> SK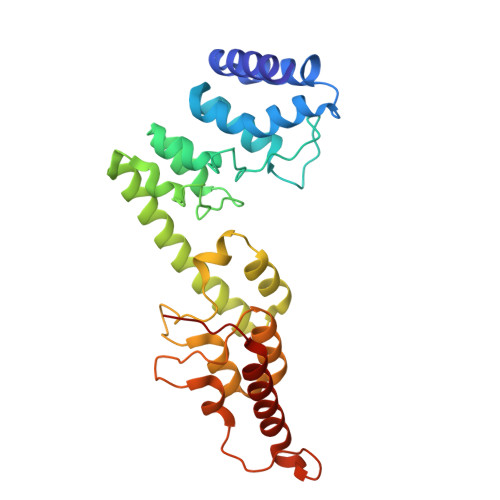PLLKLKLLDALRQGSFPNLQDLLKKQFQPLDDPNVQQVLHLMLHYAVQVAPMAVIKEIVHHWVSTTNTTFLNIHLDLNERDSNGNTPLHIAAYQSRGDIVAFLLDQPTINDCVLNNSHLQAIEMCKNLNIAQMMQVKRSTYVAETAQEFRTAFNNRDFGHLESILSSPRNAELLDINGMDPETGDTVLHEFVKKRDVIMCRWLLEHGADPFKRDRKGKLPIELVRKVNENDTATNTKIAIDIELKKLLERATREQSVIDVT> GAMDPMICLGLEGTAEKTGVGIVTSDGEVLFNKTIMYKPPKQGINPREAADHHAETFPKLIKEAFEVVDKNEIDLIAFSQGPGLGPSLRVTATVARTLSLTLKKPIIGVNHCIAHIEIGKLTTEAEDPLTLYVSGGNTQVIAYVSKKYRVFGETLDIAVGNCLDQFARYVNLPHPGGPYIEELAR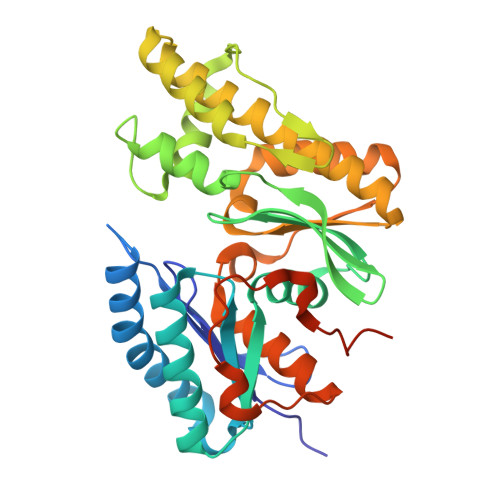KGKKLVDLPYTVKGMDIAFSGLLTAAMRAYDAGERLEDICYSLQEYAFSMLTEITERALAHTNKGEVMLVGGVAANNRLREMLKAMCEGQNVDFYVPPKEFCGDNGAMIAWLGLLMHKNGRWMSLDETKIIPNYRTDMVEVNWIKEIKGKKRKIPVEVNWIKK ethyl 5-[3-[[(2R)-4-[[[(2R,3S,4R,5R)-5-(6-aminopurin-9-yl)-4-oxidanyl-3-phosphonooxy-oxolan-2-yl]methoxy-oxidanyl-phosphoryl]oxy-oxidanyl-phosphoryl]oxy-3,3-dimethyl-2-oxidanyl-butanoyl]amino]propanoylamino]pentanoate | C26 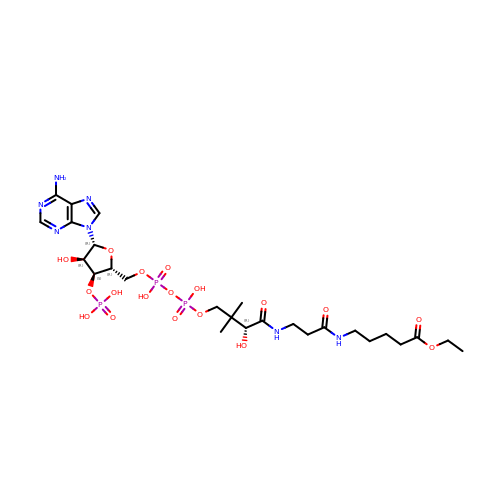H44 N7 O18 P3 | OMRRJLLNJAFEOX-ZMHDXICWSA-N> GAMGSTSLEPTSTLVRVRK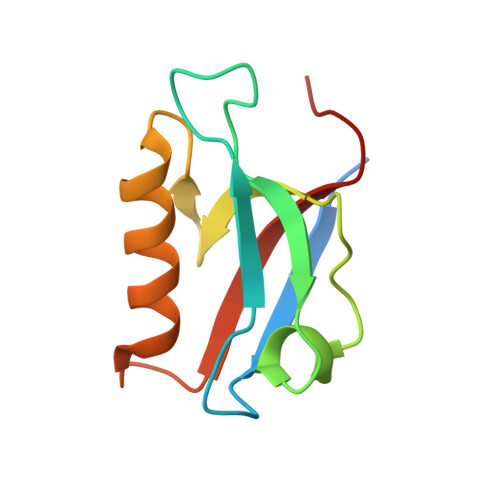SAATLGIAIEGGANTRQPLPRIVTIQRGGSAHNCGQLKVGHVILEVNGQTLRGKEHKEAARIIAEAFKTKERDYIDFLVTEFNVML>MSQAIGILELSSIAKGMELGDAMLKAANVDLLVSKTISPGKFLLMLGGDLDDIILAVAV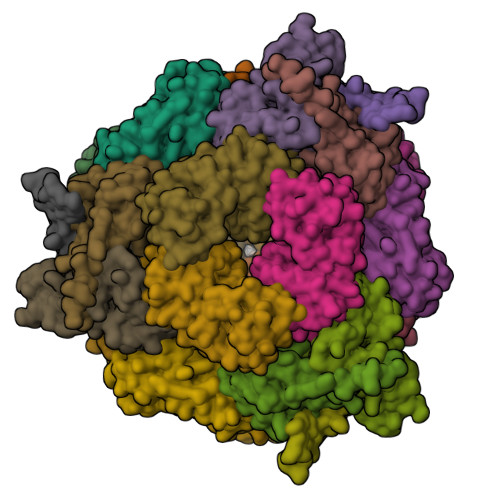GMERAGDSLLDSEVIPDIHPSVLPAISGLNSVDKRQAVGIVETWSVAACIKAADRAVKGSNVTLVRVHMAFGIGGKCYMVVAGDVSDVNNAVTVASESAGEKGLLVYRSVIPRPHEAMWRQMVEG[4x];>MTMADETIILNVLGQYTRAHDRRDPDAMAALFAPDASIVVLDAVGGASKPISVLHGRDAIRVAVRQMMAPHGYRAWSQNVVNAPVIHIHGDTARLDAQFMVFSILAAEVPDGGWPTGTFGAQGRIVPIEAGTYTLFLRTVPDGWVIAHMVIKHRLPMAFG[5x]>MSDEKVVSIGAAPLSAKEKLDLYCEGLADGLNKTQAYVAAGFSPNHAQRNVAAYHRKHSEYINAFISERIGSHVPMALRVIVSIAEDPNEKGGIRLKAAQDILDRGGFGAKQKVELTTKNVEDMSAEDLMNEVRRILDEEPDLA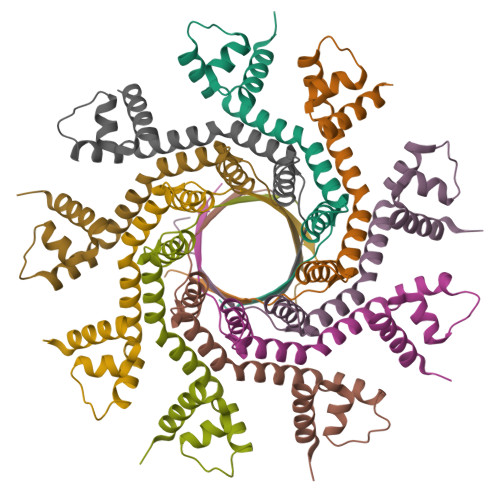KVLSFPTA[9x]> SMSLNIITVTLNMEKYNFLGISIVGQSNERGDGGIYIGSIMKGGAVAADGRIEPGDMLLQVNDMNFENMSNDDAVRVLRDIVHKPGPIVLTVAKSGGGGSTFSLWQDIP

The central event in Wnt-PCP pathway is the activation of Weak-similarity guanine nucleotide exchange factor (WGEF) by the adapter protein Dishevelled (Dvl). The PDZ domain of Dishevelled2 (Dvl2PDZ) binds and activates WGEF by releasing it from its autoinhibitory state. Dvl2PDZ binds to both C-terminal as well as the non-canonical internal peptides. Using biochemical and molecular dynamics studies, we show that a unique “internal-PDZ binding motif” (IPM) of WGEF mediates the WGEF-Dvl2PDZ interaction to activate the GEF.

The only hit, 349-GSTFSLWQDIP-359 (hereafter referred to as WGEFpep), obtained from the sequence search, lies between the DH and the inhibitory domain of hWGEF. Therefore, to obtain the structural basis of Dvl2PDZ–WGEF interaction, initially, we tried to crystallize this protein complex. Despite extensive efforts, crystallization trials met with no success. Hence, we resorted to crystallizing the WGEFpep (peptide) in complex with Dvl2PDZ. Furthermore, we tried to obtain the WGEFpep–Dvl2PDZ complex structure by fusing the peptide with the C-terminus of the PDZ domain. Due to the lack of structural information on the WGEFpep–Dvl2PDZ complex, their binding mode has remained unclear. In addition to the WGEFpep variant peptides the minimal hWGEF (330–581) construct, obtained from our solubility screening, was used for the MST study. It is interesting to note that the affinities of WGEFpep and N3pep are nearly identical for Dvl2PDZ, with dissociation constants (Kd) of 45 ± 5 and 54 ± 7 µM, respectively. Furthermore, the substitution of tryptophan (WGEFpepW7A), aspartate (WGEFpepD9A) and proline (WGEFpepP11A) residues at the P−2, P0 and P2 positions, respectively, with alanine completely abolishes the WGEF–Dvl2PDZ interactions. Compared to the other known Dvl2PDZ–internal peptide interactions, in the WGEF-Dvl2PDZ complex, only five residues at the P2, P0, P−1, P−2 and P−3 positions appear to contribute significantly in stabilizing their interactions.>[2x]GSWSGGSGGEAADEARRAIEAALEEARAAADEARSDSTGETVKKAVDKAEKAAEDAFREIKQAVNQAEKQGASEAAFEAFAAIAAAAAEAAAAAFEAFSDSTGETVAEAVAKALKAAMEAFAEIAKAVAQAAKQGA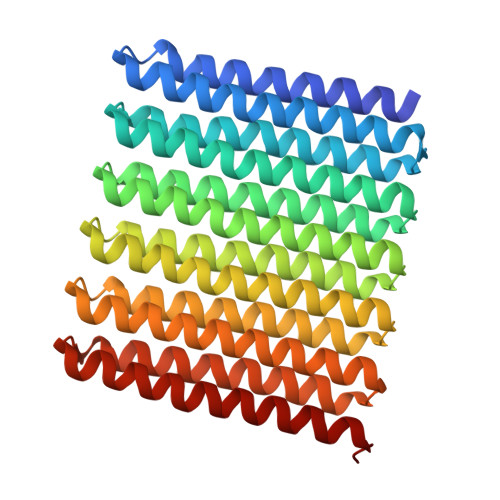SEAAFEAFAAIAAAAAEAAAAAFEAFSDSTGETVAEAVAKALKAAMEAFAEIAKAVAQAAKQGASEAAFEAFAAIAAAAAEAAAAAFEAFSDSTGETVAEAVAKALKAAMEAFAEIAKAVAQAAKQGASEAAFEAFAAIAAAAAEAAAAAFEAFSDSTGETVAEAVAKALKAAMEAFAEIAKAVAQAAKQGASEEAFEKFAAIAAEAAEAAAAAFERFSDSTGETEAEKVAKELKQLMEEFAERAKSVAEQAKNGAS>[2x]MFSAGHKIKGTVVLMPKNELEVNPDGSAVDNLNAFLGRSVSLQLISATKADAHGKGKVGKDTFLEGINTSLPTLGAGESAFNIHFEWDGSMGIPGAFYIKNYMQVEFFLKSLTLEAISNQGTIRFVCNSWVYNTKLYKSVRIFFANHTYVPSETPAPLVSYREEELKSLRGNGTGERKEYDRIYDYDVYNDLGNPDKSEKLARPVLGGSSTFPYPRRGRTGRGPTVTDPNTEKQGEVFYVPRDENLGHLKSKDALEIGTKSLSQIVQPAFESAFDLKSTPIEFHSFQDVHDLYEGGIKLPRDVISTIIPLPVIKELYRTDGQHILKFPQPH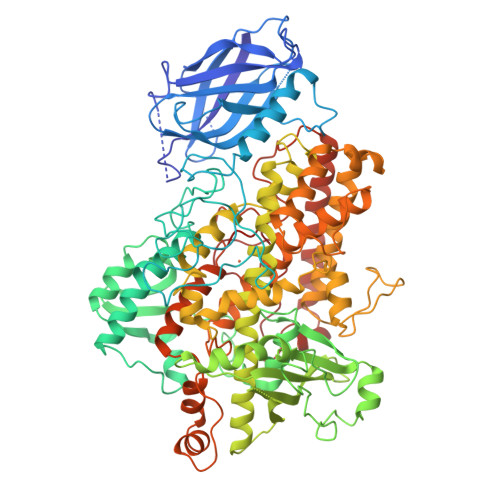VVQVSQSAWMTDEEFAREMIAGVNPCVIRGLEEFPPKSNLDPAIYGDQSSKITADSLDLDGYTMDEALGSRRLFMLDYHDIFMPYVRQINQLNSAKTYATRTILFLREDGTLKPVAIELSLPHSAGDLSAAVSQVVLPAKEGVESTIWLLAKAYVIVNDSCYHQLMSHWLNTHAAMEPFVIATHRHLSVLHPIYKLLTPHYRNNMNINALARQSLINANGIIETTFLPSKYSVEMSSAVYKNWVFTDQALPADLIKRGVAIKDPSTPHGVRLLIEDYPYAADGLEIWAAIKTWVQEYVPLYYARDDDVKNDSELQHWWKEAVEKGHGDLKDKPWWPKLQTLEDLVEVCLIIIWIASALHAAVNFGQYPYGGLIMNRPTASRRLLPEKGTPEYEEMINNHEKAYLRTITSKLPTLISLSVIEILSTHASDEVYLGQRDNPHWTSDSKALQAFQKFGNKLKEIEEKLVRRNNDPSLQGNRLGPVQLPYTLLYPSSEEGLTFRGIPNSISI>UGGAAGAAAUCGAAGAAGAUGAAGAACGCGAAGAAC[2x];>[2x]AUCUUCUUCGAUUUCUUCCAGUUCUUCGCGUUCUUC

Recently, RNA-catalyzed rolling circle synthesis (RCS) on small circular RNA (scRNA) templates has been demonstrated. To gain deeper insight into the RCS process and the strong inhibition observed upon full-length circle synthesis, we used cryo-EM to study the structure of putative RCS replication products formed by complexing the full-length scRNA and nascent complementary RNA (cmpRNA). To our surprise, cryo-EM revealed not one by a diverse variety of distinct structural species identified as monomers, dimers, and multimers of the scRNA–cmpRNA complex. We find that scRNAs and cmpRNAs of 36 nt in length can form an unanticipated diversity of structures with different stoichiometries, including a fully annealed dimer (comprising two scRNAs and two cmpRNAs) and multimers hereof.

Class 3 led to our best-resolved structure showing two parallel helixes, each having slightly >3 helical turns. Based on the identified structures, we concluded that class 3 likely represents a homodimer between two scRNA–cmpRNA complexes that have dimerized by strand exchange and mutual cross-hybridization. The dimer from class 3 was found to be composed of two scRNAs and two cmpRNAs that are fully hybridized. The cryo-EM reconstruction using C2 symmetry led to our highest resolution map of 5.3 Å. Based on this map, we built an atomic model, which fitted the density well consisting of two parallel RNA helices of 36 bp connected by anti-parallel crossovers formed by the two scRNAs—a central two-strand crossover and two proximal one-strand crossovers (see Supplementary Fig. S7 for comparing C1 and C2 symmetries). A nonideal crossover spacing is observed, with 22 bp on one helix and 14 bp on the other. The nonideal crossover length of the 14-bp segment results in its underwinding and a global distortion of the structure where the 22-bp helix bends outward and the 14-bp segment bends inward giving the structure a slightly curved shape. The model suggests that the central crossover in the dimer forms a C2′-endo conformation adopted by the nucleotide at the 5′-end of the strand entering the crossover. The distortion of the helices results in bringing the 5′- and 3′-ends of the two different cmpRNAs into close proximity, with the 5′-end of one cmpRNA projecting above the 3′-end of the other cmpRNA. The structure of the class 3 dimer suggests that it may act as a dead-end product for RCS by inhibiting 3′-end extension due to its thermodynamic stability and poor accessibility of 3′-ends, providing a plausible candidate for the previously observed full-length synthesis inhibition.> GPSQPKVPEWVNTPSTCCLKYYEKVLPRRLVVGYRKALNCHLPAIIFVTKR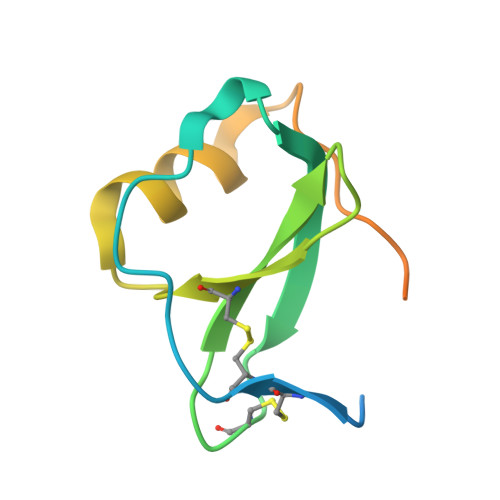NREVCTNPNDDWVQEYIKDPNLPLLPTRNLSTVKIITAKNGQPQLLNSQ>[2x]DVQKKTFTKWINARFSKSGKPPINDMFTDLKDGRKLLDLLEGLTGTSLPKERGSTRVHALNNVNRVLQVLHQNNVELVNIGGTDIVDGNHKLTLGLLWSIILHW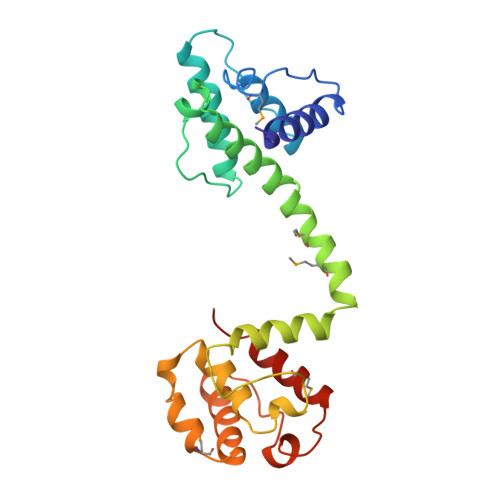QVKDVMKDVMSDLQQTNSEKILLSWVRQTTRPYSQVNVLNFTTSWTDGLAFNAVLHRHKPDLFSWDKVVKMSPIERLEHAFSKAQTYLGIEKLLDPEDVAVRLPDKKSIIMYLTSLFEVLPQ>GPLGSMINAKTKVIGLIGHPVEHSFSPIMHNAAFKDKGLNYVYV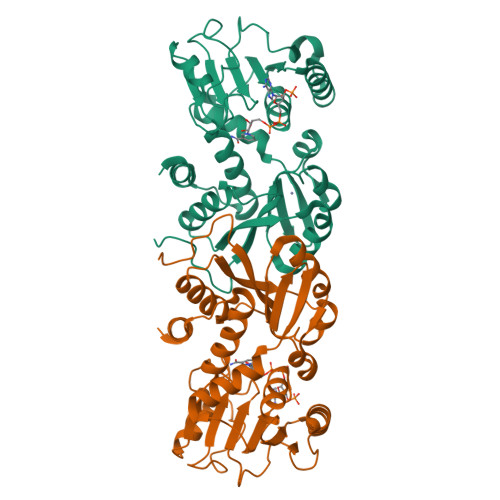AFDVLPENLKYVIDGAKALGIVGFNVTIPHKIEIMKYLDEIDKDAQLIGAVNTIKIEDGKAIGYNTDGIGARMALEEEIGRVKDKNIVIYGAGGAARAVAFELAKDNNIIIANRTVEKAEALAKEIAEKLNKKFGEEVKFSGLDVDLDGVDIIINATPIGMYPNIDVEPIVKAEKLREDMVVMDLIYNPLETVLLKEAKKVNAKTINGLGMLIYQGAVAFKIWTGVEPNIEVMKNAIIDKITK[2x]> M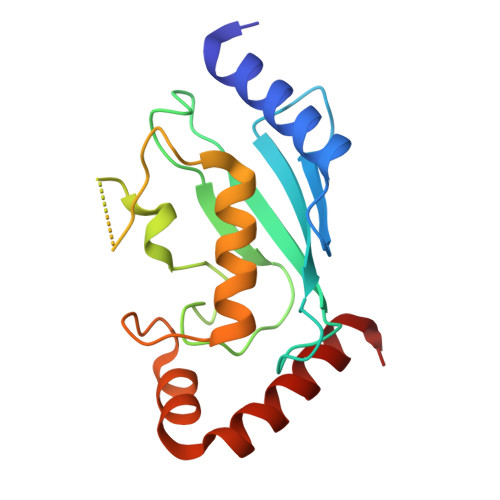AGTALKRLMAEYKQLTLNPPEGIVAGPMNEENFFEWEALIMGPEDTCFEFGVFPAILSFPLDYPLSPPKMRFTCEMFHPNIYPDGRVCISILHAPGDDPMGYESSAERWSPVQSVEKILLSVVSMLAEPNDESGANVDASKMWRDDREQFYKIAKQIVQKSLGL1-(pyridin-4-yl)methanamine | C6 H8 N2 | 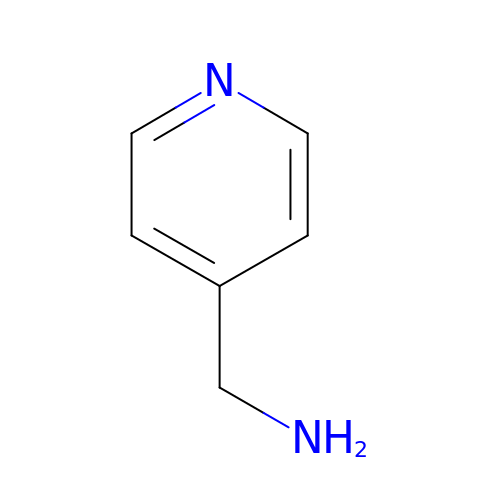TXQWFIVRZNOPCK-UHFFFAOYSA-N> GRAPDSVDYRKKGYVTPVKNQGQCGSCWAFSSVGALEGQLKKKTGKLLNLSPQNLVDCVSENDGCGGGYMTNAFQYVQKNRGIDSEDAYPYVGQEESCMYNPTGKAAKCRGYREIPEGNEKALKRAVARVGPVSVAIDASLTSFQFYSKGVYYDESCNSDNLNHAVLAVGYGIQKGNKHWIIKNSWGENWGNKGYILMARNKNNACGIANLASFPKM

Cathepsin K (CatK) is one of the most investigated cysteine cathepsins, both by academia and pharmaceutical companies. It is expressed in high levels in osteoclasts, where it serves as the principal protease involved in bone remodelling. Cathepsin K (CatK) is a target for the treatment of osteoporosis, arthritis, and bone metastasis. Peptidomimetics with a cyanohydrazide warhead represent a new class of highly potent CatK inhibitors; however, their binding mechanism is unknown.

The final crystallographic models contained mCatK residues Ala1 to Met215; additional N-terminal residues derived from the propeptide, Gly-Arg (98p–99p, propeptide numbering), were visible in the mCatK-Gü1303 structure. The active site cleft of mCatK contains the catalytic triad residues Cys25, His162, and Asn182. Gü1303 is bound in a substrate-like orientation, and its P1 to P3 residues occupy the S1 to S3 subsites of mCatK (Figure 4(A,C)). The cyanohydrazide warhead reacts with the thiol group of the catalytic Cys25, forming a covalent isothiosemicarbazide adduct through the connection to the C-atom of the nitrile moiety. However, a Z-configuration at the CO–NMe bond was observed in Gü1303 bound to mCatK, suggesting an E- to Z-conformational change in Gü1303 upon binding to the enzyme, most likely due to a "configurational selection" that we recently reported for an azadipeptide nitrile inhibitor of the protease SmCB1. The nitrogen atom of the imidate moiety, derived from the warhead nitrile group, is stabilised by two hydrogen bonds to the backbone amide of the catalytic Cys25 and the side chain amide of Gln19. The NH of Gly66 acts as a bifurcated hydrogen bond donor for the carbonyl oxygen of the P2 phenylalanine and the noncarbonyl carbamate oxygen in the P3 position of Gü1303. An additional hydrogen bond is formed between the Gly66 oxygen and the carbamate NH of Gü1303. At the P2 position, the phenylalanine residue makes nonpolar interactions with Tyr67, Ala134, Leu160, Ala163, and Leu209. The P3 benzyloxycarbonyl capping group forms nonpolar interactions with Asp61 and Tyr67, and the phenyl moiety of this group is stabilised by a T-shaped π-π stacking interaction to the 4-hydroxyphenyl group of Tyr67. Gü1303 occupies the non-primed subsites S1 to S3, and B-factor distribution showed that Gü1303 is rigid in the mCatK active site.>[8x]MSLTNHHPSSTGPQHPYRAGWIHFTNVAPILDSLELPPGVTAITGVPTQMNAALLSGEVDIANVSAVEFIRHADTLAALPDFSVAVLGPVYSVNLFHTCPLPELRRVALTSQSAMSVALLEVLLRQKGLSPVLERAEGTAESLLAAGYDGVLRIGDDALREWYGVVGPLTPERTMTSLPHTGRGITVTDLAQEWFDLTGHPFTFAVWAYRKDN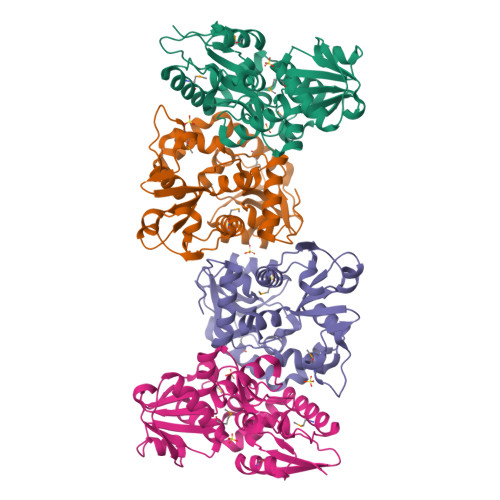PPPAALLQAMREARRRGIGHLAEVSQRHAEKLGLPERVVQHYLWNFRYHLEAPDRLGLREFADLAVPGHAELTFGAREEAEGHHHHHH>[2x]MNYLFKNGRYMNEEGKIVATDLLVQDGKIAKVAENITADNAEVIDVNGKLIAPGLVDVHVHLREPGGEHKETIETGTLAAAKGGFTTICAMPNTRPVPDCREHMEDLQNRIKEKAHVNVLPYGAITVRQAGSEMTDFETLKELGAFAFTDDGVGVQDASMMLAAMKRAAKLNMAVVAHCEENTLINKGCVHEGKFSEKHGLNGIPSVCESV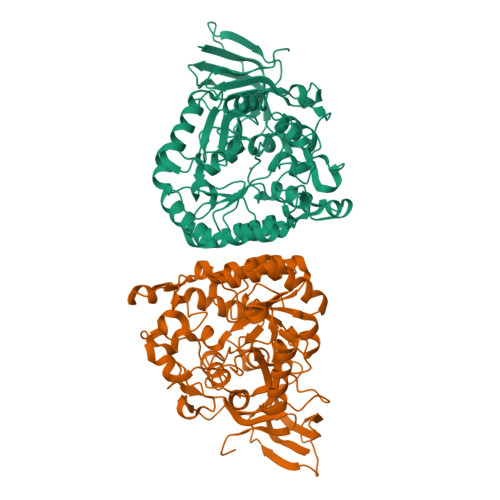HIARDILLAEAADCHYHVCHVSTKGSVRVIRDAKRAGIKVTAEVTPHHLVLCEDDIPSADPNFKMNPPLRGKEDHEALIEGLLDGTIDMIATDHAPHTAEEKAQGIERAPFGITGFETAFPLLYTNLVKKGIITLEQLIQFLTEKPADTFGLEAGRLKEGRTADITIIDLEQEEEIDPTTFLSKGKNTPFAGWKCQGWPVMTIVGGKIAWQKESALV> PGPVPPSTAVRELIEELINITQNQKAPLCNGSMVWSINRTAGMYCAALESLINVSGCSAIEKTQRMLSGFCPHKVSAGQFSSLHVRSSKIEVAQFVKDLLFHLRTLFREGQFN;> MKVLQEPTCVSDYMSISTCEWKMNGPTNCSTELRLLYQLVFLLSEAHTCIPENNGGAGCVCHLLMDDVVSADNYTLDLWAGQQLLWKGSFKPSEHVKPRAPGNLTVHTNVSDTLLLTWSNPYPPDNYLYNHLTYAVNIWSENDPADFRIYNVTYLEPSLRIAASTLKSGISYRARVRAWAQCYNTTWSEWSPSTKWHNSYREP;> GGGAAPTETQPPVTNLSVSVENLCTVIWTWNPPEGASSNCSLWYFSHFGDKQDKKIAPETRR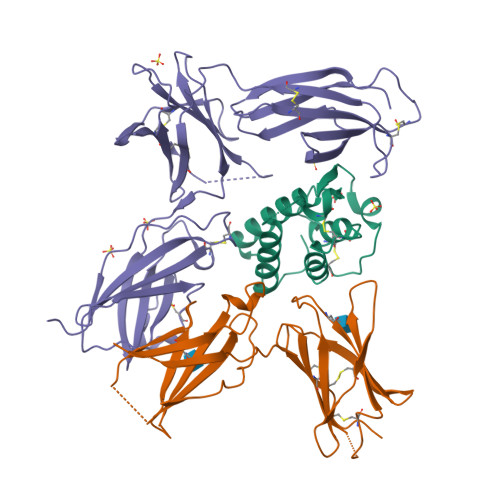SIEVPLNERICLQVGSQCSTNESEKPSILVEKCISPPEGDPESAVTELQCIWHNLSYMKCSWLPGRNTSPDTNYTLYYWHRSLEKIHQCENIFREGQYFGCSFDLTKVKDSSFEQHSVQIMVKDNAGKIKPSFNIVPLTSRVKPDPPHIKNLSFHNDDLYVQWENPQNFISRCLFYEVEVNNSQTETHNVFYVQEAKCENPEFERNVENTSCFMVPGVLPDTLNTVRIRVKTNKLCYEDDKLWSNWSQEMSIGKKR>[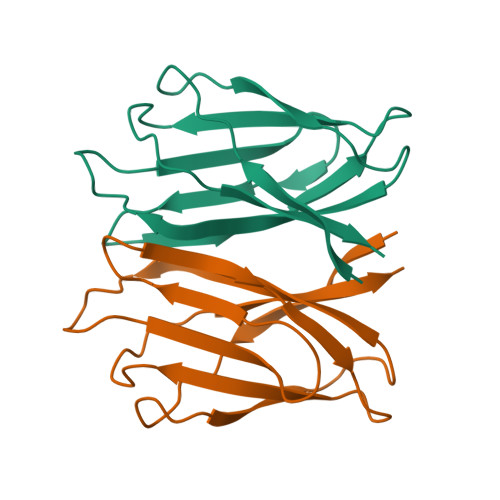4x]NPTSLTDVRVDKAVNFIKPEVSGVAEIQTVTGLSPSTSYLLTPAFLEQNFQSEAGIYILSATPVEGEGTISINMDPTVTTVSGFIKVKTDTFGTFDLSVVLTTASKKQTTGFNIIAATS>MDVFAKHAVSLESPAVRHYEITPSDSTDLARRPRALRVQTGGTLVLRDETGITVTYTVFAGEILPVRPVRVLATGTTATAVGWE[11x];>MPEGADPVAEVKTALAGFLKEVKGFQDDVKTRLQQQEERVTMLQTKTYAGRHALAAAATEEAPHQKAFAAYLRTGDDDGLRGLSLEGKALNSAVAAEGGYLVDPQTSETIRGVLRSTASLRQIASVVNVEATSFDVLVDKTDMGSGWASETAALSETATPQIDRITIPLHELAAMPKASQRLLDDSAFDIETWLANRIADKFARAEAAAFISGDGVDKPTGFLTKTKVANGAWAWGSLGYVATGAAGDFAAVNASDAVVDLVYALGAEYRANASFVMNSKTAGAVRKMKDADGRFLWADSLAAGEPARLMGYPVLIAEDMPDIAANAYAIAFGDFGNGYTIAERPDLRVLRDPFSAKPHVLFYASKRVGGDVSDFAAIKLLKFAAS[29x];>[2x]MIALGLGLGLAANGGPALRRYAVNGVAPVAVLDFERHFLSHPLALTRATSATYADALRAVQTAPADTPRYDYSTGKRALLLEASATNLLPNSAQFEAASWGKTRASVLANAALAPNGTMTADKLVEDTSNNSHFVARTGTQIAAGTSVTASIFVKAAERRWFALVTADSANAFRTTYFDLQTGTLGVVSQGAAGHVAQIVAAGNGWYRCSVTQTQAASGNFNFYPSVASANGATSYPGDGASGLYLWGAQLEAGAAVSSVIPTEAAAVTRAADLASVAVAAGSYDLRRVDAAGTAVTKGVAHPGGALTIGAGSLYLLSLFPAGAL

Gene transfer agents (GTAs) are DNA-containing phage-like particles produced by some species of bacteria and archaea. The genes encoding proteins that form Rhodobacter capsulatus GTA particles (RcGTA) are derived from phage DNA, which has been integrated into the bacterial genome. Here, we use cryo-electron microscopy (cryo-EM) to determine the structures of RcGTA before and after DNA ejection, and to visualize the interactions of RcGTA with R. capsulatus cells. Particles of RcGTA have heads with a diameter of 38-nm and 49-nm long tails.

Unlike the phage heads that are isometric or prolate, the capsid of RcGTA is oblate with the shortened dimension along the tail axis. The organization of the RcGTA capsid is derived from a T = 3 quasi-icosahedral lattice; however, it lacks five hexamers of major capsid proteins in its central part, which results in a shortening of the head. By contrast, the quasi-hexamers on twofold axes of the oblate capsid are bent to enable seamless closure of the oblate head. The quasi-hexamers on twofold axes of the oblate head contain subunits in three conformations: two subunits binding to pentamers from different directions, and one binding to a hexamer of capsid proteins. The surface of the RcGTA head is decorated with eleven 70-Å long head spikes attached to pentamers of major capsid proteins. Each head spike is composed of a pentamer of base proteins Rcc01079, and a single subunit of head fiber protein Rcc01080. Base proteins attach to the capsid by the N-termini, each of which binds to axial domains of two adjacent major capsid proteins within a pentamer. The attachment is reinforced by the coordination of a cation.>[2x]MDVSFRLSGATSSSYGVFISNLRKALPNERKLYDIPLLRSSLPGSQRYALIHLTNYADETI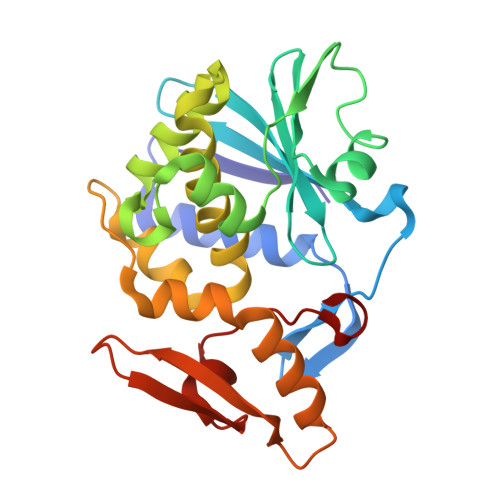SVAIDVTNVYIMGYRAGDTSYFFNEASATEAAKYVFKDAMRKVTLPYSGNYERLQTAAGKIRENIPLGLPALDSAITTLFYYNANSAASALMVLIQSTSEAARYKFIEQQIGAAVDATFLPSLAIISLENSWSALSKQIQIASTNNGQFESPVVLINAQNQRVTITNVDAGVVTSNIALLLNRNNMA>MSQASSTDTPFVIAGRTYGSRLLVGTGKYKDLDETRRAIEASGAEIVTVAVRRTNIGQNPDEPNLLDVIPPDRYTILPNTAGCYDAVEAVRTCRLARELLDGHNLVKLEVLADQ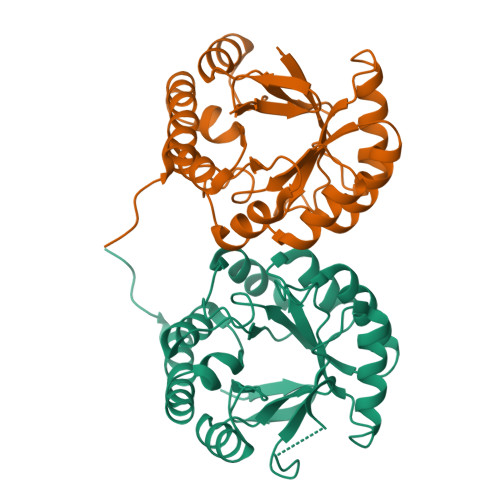KTLFPNVVETLKAAEQLVKDGFDVMVYTSDDPIIARQLAEIGCIAVMPLAGLIGSGLGICNPYNLRIILEEAKVPVLVDAGVGTASDAAIAMELGCEAVLMNTAIAHAKDPVMMAEAMKHAIVAGRLAYLAGRMPRKLYASASSPLDGLID[2x]>MTGNLVTKNSLTPDVRNGIDFKIADLSLADFGRKELRIAEHEMPGLMSLRREYAEVQPLKGARISGSLHMTVQTAVLIETLTALGAEVRWASCNIFSTQDHAAAAVVVGPHGTPDEPKGVPVFAWKGETLEEYWWAAEQMLTWPDPDKPANMILDDGGDATMLVLRGMQYEKAGVVPPAEEDDPAEWKVFLNLLRTRFETDKDKWTKIAESVKGVTEETTTGVLRLYQFAAAGDLAFPAINVNDSVTKSKFDNKYGTRHSLIDGINRGTDALIGGKKVLICGYGDVGKGCAEAMKGQGARVSVTEIDPINALQAMMEGFDVVTVEEAIGDADIVVTATGNKDIIMLEHIKAMKDHAILGNIGHFDNEIDMAGLERSGATRVNVKPQVDLWTFGDTGRSI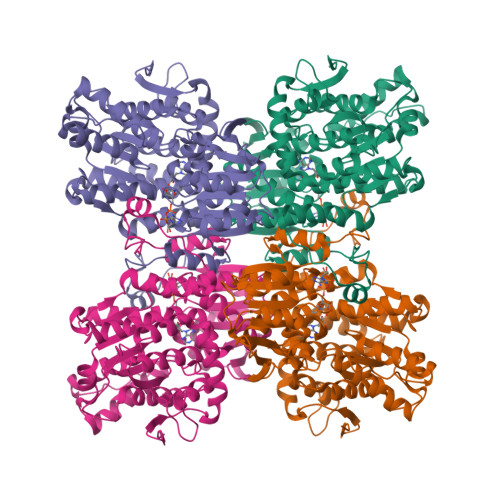IVLSEGRLLNLGNATGHPSFVMSNSFANQTIAQIELWTKNDEYDNEVYRLPKHLDEKVARIHVEALGGHLTKLTKEQAEYLGVDVEGPYKPDHYRY[4x]>[4x]MSVGIVYGDQYRQLCCSSP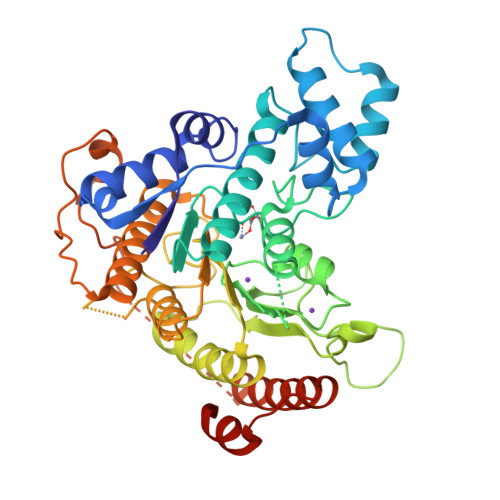KFGDRYALVMDLINAYKLIPELSRVPPLQWDSPSRMYEAVTAFHSTEYVDALKKLQMLHCEEKELTADDELLMDSFSLNYDCPGFPSVFDYSLAAVQGSLAAASALICRHCEVVINWGGGWHHAKRSEASGFCYLNDIVLAIHRLVSSTPPETSPNRQTRVLYVDLDLHHGDGVEEAFWYSPRVVTFSVHHASPGFFPGTGTWNMVDNDKLPIFLNGAGRGRFSAFNLPLEEGINDLDWSNAIGPILDSLNIVIQPSYVVVQCGADCLATDPHRIFRLTNFYPNLNLDSDCDSECSLSGYLYAIKKILSWKVPTLILGGGGYNFPDTARLWTRVTALTIEEVKGKKMTISPEIPEHSYFSRYGPDFELDIDYFPHESHNKTLDSIQKHHRRILEQLRNYADLNKLIYDYDQVYQLYNLTGMGSLVPR> SAKDPNISFIDNTKLELQNGDEFLFIGDSLMQGVAIALNRDLRNLNLKVTDLSKQNTGLSYKSYFDWSKATNEAFIKNSNIKYLVVLLGANDPW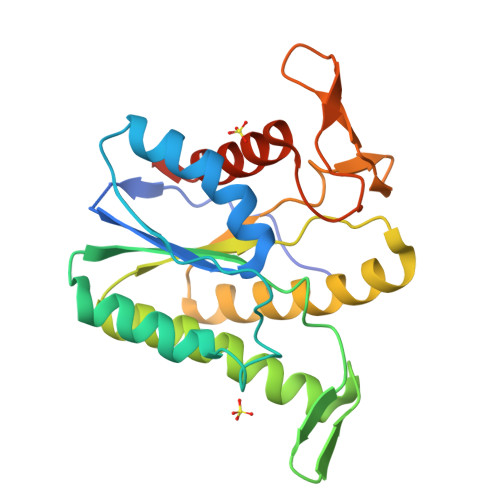DIKKGGNYHRFGSPSWIDIYTSRVDEIIKIAKKHKAKVFWFEIPPVKKEDLNKKIQVLNKIYSDEILKNKEIFINTKLFFSVNDEYSAYIKDENNRSIKVRTDDGVHFTPSGAREMSKLLLEHIKLKEENASK>[2x]MDTPNKDDSIIRFSVSLQQNLLDELDNRIIKNGYSSRSELVRDMIREKLVEDNWAEDNPNDESKIAVLVVIYDHHQ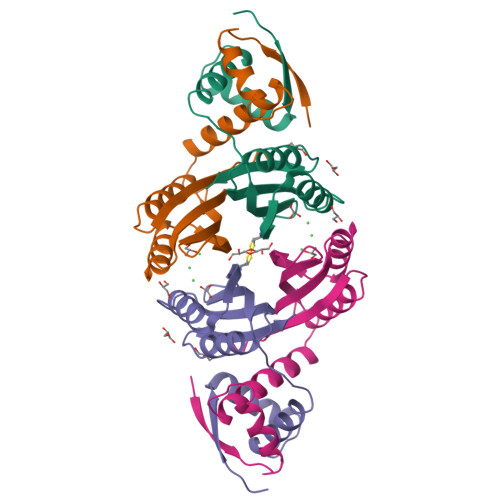RELNQRMIDIQHASGTHVLCTTHIHMDEHNCLETIILQGNSFEIQRLQLEIGGLRGVKFAKLTKASSFEYNE>[2x]MKHHHHHHSAGLEVLFQGPRRQTIEALVPAWDSDIIFKCLCYFHTLYPGLIPLETFPPATIFNFKQKIISILEDKKAVLRGEPIKG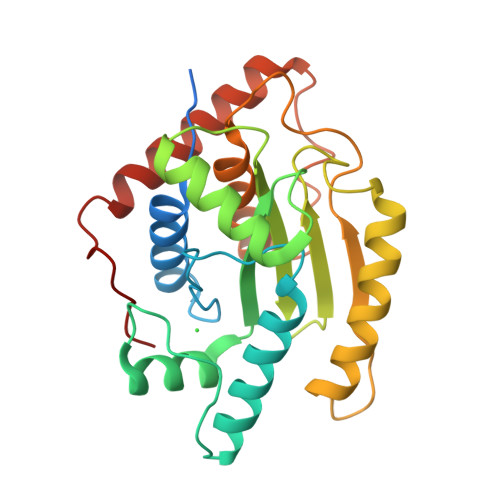PLPICCSKENYRRHLQRTTLLPVFMWYHPTPKTLSDTMQTMKQLAIKGSVGASHWLLVIVDIQARRLVYFDSLYNYVMPPENMKKELQSFAQQLDQVYPAYDSKKFSVKIAAKEVIQRGSGSSCGAWCCQFLHWYLKDPLTDALNDLPVDSVERHENLASFVQACEAAVQDLPELSWPEA>[4x]GVTSDTVFVRETQIPILIERQDNVLFMLRLNAKESRSLDEVVLNFGKDVNMADI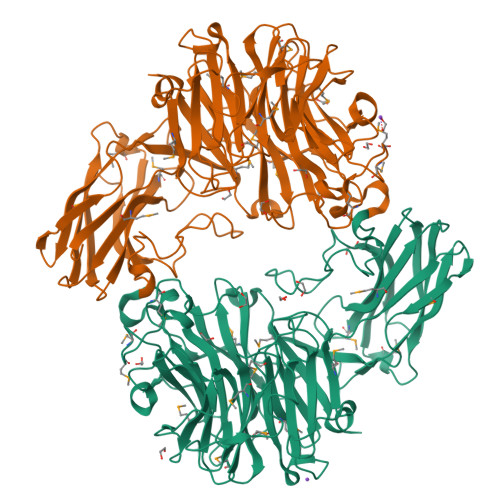QSVKLYYSGTEARQNYGKKFFTPVSYISSHTPGKTLAANPSYSINKSQVNNPGRKVILNANQKLFPGINYFWISLQMKPGASLLDKVSAKIVTVKVDNKEALMHTVSPENIAHRVGVGVRHAGDDGSAAFRIPGLATTNKGTLLGVYDVRYNSSVDLQEHVDVGLSRSVDGGKTWEKMRLPLAFGETGGLPAAQNGVGDPSILVDTKTNTTWVVAAWTHGMGNQRAWWSSYPGMDMNHTAQLVLSKSTDDGKTWSEPINITDQVKDPSWYFLLQGPGRGITMQDGTLVFPIQFIDSTRVPNAGIMYSKDRGETWKIHNYARTNTTEAQVAEVEPGVLMLNMRDNRGGSRAVATTKDLGKTWTEHPSSRKALQEPVCMASLISVKAADNTLNKDILLFSNPNTVKGRHHITIKASLDGGITWLPEHQVMLDEGDGWGYSCLTMIDKETVGILYESSVAHMTFQAIRLRDIIQ>SMSRITIERDGLTLVGDREEPFGEIYDMAILMHGFTANRNTPLLRQIADNLRDENVASVRFDFNGHGESDGAFEDMTVCNEIADAQKILEYVRTDPHVRNIFLVGHSQGGVVASMLAGLYPDIVKKVVLLAPA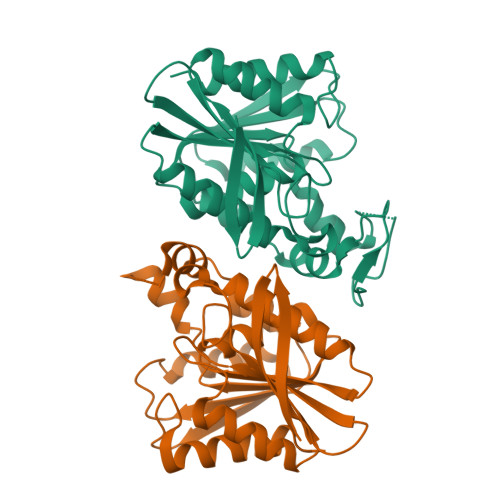AQLKDDALNGDTQGATYNPEHIPAAIPFHGKKLGGFYLRTAQVLPIYEIAKHYTNPVSIIVGSNDQVVAPKYSKKYDEVYENSELHMVPDADHSFTGQYKDSAVDLTAEFLKPLF[2x]>[2x]MGPAFDITVVIPTFKAEKTVGQCLESVLSQQGVSTEIIVVDGGSPDATISIVQSFSSTNLTIISEPDRGIYDAINKGVSRAQGGMIGVLGADDVYKPNVLSVVKENASRGVEIVAGLTLIDGQLRADEQYRPAALISGIPFGHNAMFASQEAYRKVG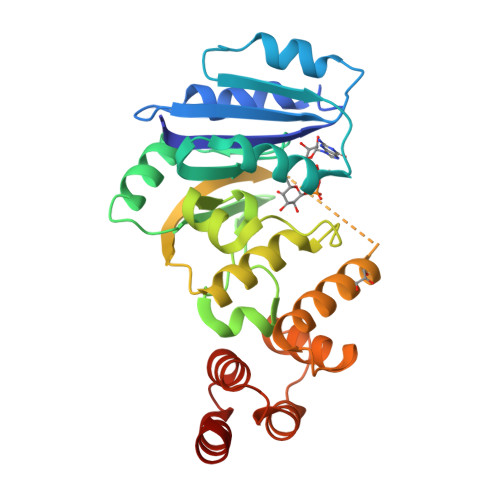LYDLAYRICADAEWVHRAIKSDISCRKVEQVFVEFGTEGTSSTNPEEIIAEACSVIQRNFPFLLKEEAKYLLYGVRGWGETSRIEQILRKYGHESVLFVTALQEAFPAVETAAALEHHHHHH(2R)-4-[(8R)-8-METHYL-2-(TRIFLUOROMETHYL)-5,6-DIHYDRO[1,2,4]TRIAZOLO[1,5-A]PYRAZIN-7(8H)-YL]-4-OXO-1-(2,4,5-TRIFLUOROPHENYL)BUTAN-2-AMINE 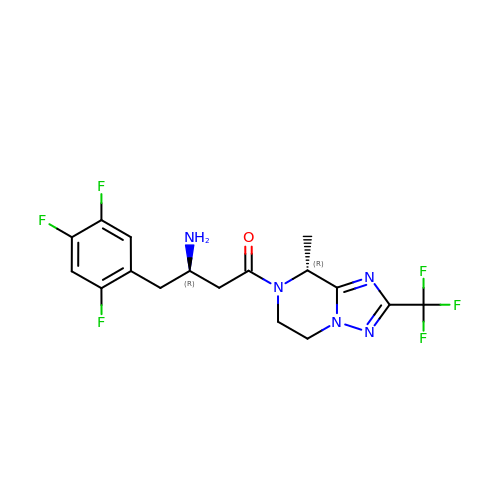| C17 H17 F6 N5 O | FDEXEPZGMKFCTG-PSASIEDQSA-N> KKIKLNIKEFKATAEGLSPEEKELWDKFAEKLKAELNNKIINLGEKIEIEEELKTPTKSIKITFSLELVSEDTFKATLKLEIKGKETIVE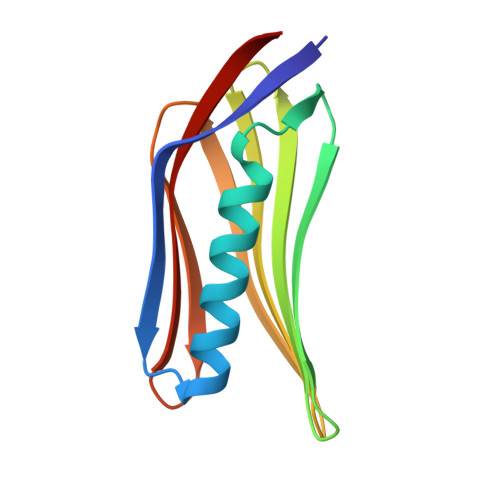EETVEFKAGETVKLTIKLPDGKTFTLELKLEATKI>MTISRRDFLNGVALTIAAGLTPAEILRAAPGGRYYPPALTGLRGSHPGAFEVAHQMGWEKKTFDVDHLPIEEEYDLVVVGGGISGLAAAWFYRERHPAARILVIENHDDFGGHAKRNEFQAGGRTILGYGGSESLQSPNALYSEDAKHLLKRLGVELKRFETAFDTDFYPGLGLSRAVFFDKASFGVDKLVSGDPTPMVADEVPRDRLNARSWRAFIGDFPLSREDREALIALYESPRDYLAGKSVEEKETYLAKTSYRDYLLKNVGLSETSVKYFQGRSNDFSALGADALPAADAYAAGFPGFDALGLPQPSEEAQAEMDEPYIYHFPDGNASLARLMVRDLIPAVAPGRGMEDIVMARFDYSKLDLAGHPVRLRLNSTAVSVRNRAGGVDVGYSRAGRLHRVRGKHCVMACYNMMVPYLLRDLSEEQAHALSQNVKFPLVATKVLLRNWQAWKTLGIHEIYAPTLPYSRIKLDFPVDLGSYRH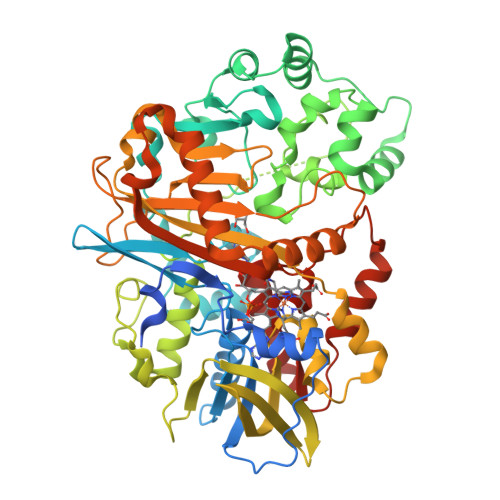PRDPRQPIGVHMVYVPTTPNAGMDARTQARVGRSKLYAMSFEQLEKDIRDQLQAMLGPAGFDHRRDITGITVNRWSHGYSYFMNTLYDDEAESEALMELARSKVGNVAIANSDAAWDAYAHAAIDQAVRAVRELG[2x]>[2x]MGSSHHHHHHSQDPAEKQKHDGRVKIGHYVLGDTLGVGTFGKVKIGEHQLTGHKVAVKILNRQKIRSLDVVGKIKREIQNLKLFRHPHIIKLYQVISTPTDFFMVMEYVSGGELFDYICKHGRVEEMEARRLFQQILSAVDYCHRHMVVHRDLKPENVLLDAHMNAKIADFGLSNMMSDGEFLRTSCGSPNYAAPEVISGRLYAGPEVDIWSCGVILYALLCGTLPFDDEHVPTLFKKIRGGVFYIPEYLNRSVATLLMHMLQVDPLKRATIKDIREHEWFKQGLPSYLFPEDPSYDANVIDDEAVKEVCEKFECTESEVMNSLYSG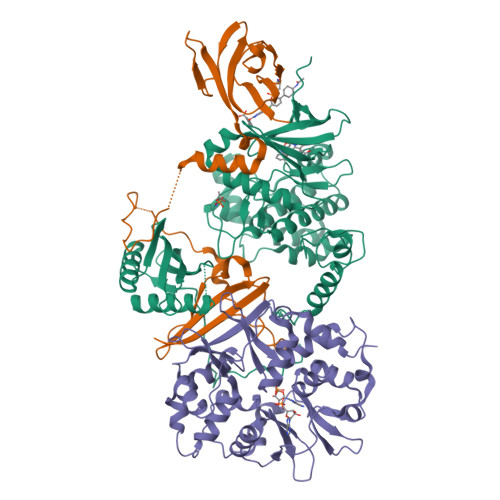DPQDQLAVAYHLIIDNRRIMNQASEFYLASSPPSGSFMDDSAMHIPPGLKPHPERMPPLIADSPKARCPLDALNTTKPKSLAVKKAKWHLGIRSQSKPYDIMAEVYRAMKQLDFEWKVVNAYHLRVRRKNPVTGNYVKMSLQLYLVDNRSYLLDFKSIDDEVVEQRSGSSTPQRSCSAAGLHRPRSSFDSTTAESHSLSGSLTGSLTGSTLSSVSPRLGSHTMDFFEMCASLITTLAR;>[2x]MGNTSSERAALERHGGHKTPRRDSSGGTKDGDRPKILMDSPEDADLFHSEEIKAPEKEEFLAWQHDLEVNDKAPAQARPTVFRWTGGGKEVYLSGSFNNWSKLPLTRSHNNFVAILDLPEGEHQYKFFVDGQWTHDPSEPIVTSQLGTVNNIIQVKKTDFEVFDALMVDSQKCSDVSELSSSPPGPYHQEPYVCKPEERFRAPPILPPHLLQVILNKDTGISCDPALLPEPNHVMLNHLYALSIKDGVMVLSATHRYKKKYVTTLLYKPI;>[2x]MADLNWETVISSDSSPAVENEHPQETPESNNSVYTSFMKSHRCYDLIPTSSKLVVFDTSLQVKKAFFALVTNGVRAAPLWDSKKQSFVGMLTITDFINILHRYYKSALVQIYELEEHKIETWREVYLQDSFKPLVCISPNASLFDAVSSLIRNKIHRLPVIDPESGNTLYILTHKRILKFLKLFITEFPKPEFMSKSLEELQIGTYANIAMVRTTTPVYVALGIFVQHRVSALPVVDEKGRVVDIYSKFDVINLAAEKTYNNLDVSVTKALQHRSHYFEGVLKCYLHETLETIINRLVEAEVHRLVVVDENDVVKGIVSLSDILQALVLTGGEKKP>[2x]GADSVKIGFITDMSGLYADIDGQGGLEAIKMAVADFGGKVNGKPIEVVYADHQNKADIAASKAREWMDRGGLDLLVGGTNSATALSMNQVAAEKKKVYINIGAGADTLTNEQCTPYTVHYAYDTMALAKGTGSAVVKQGGKTWFFLTADYAFGKALEKNTADVVKANGGKVLG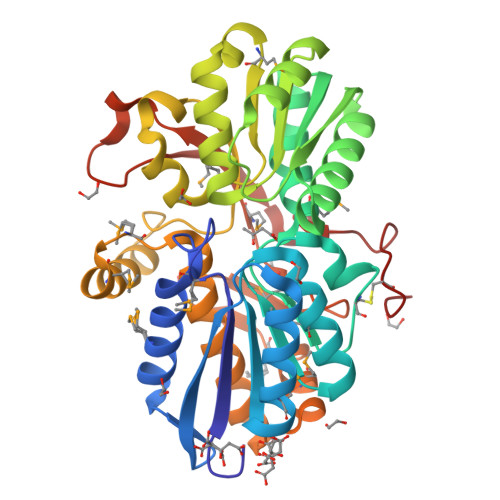EVRHPLSASDFSSFLLQAQSSKAQILGLANAGGDTVNAIKAAKEFGITKTMKLAALLMFINDVHALGLETTQGLVLTDSWYWNRDQASRQWAQRYFAKMKKMPSSLQAADYSSVTTYLKAVQAAGSTDSDKVMAQLKKMKIDDFYAKGYIRTDGSMIHDMYLMEVKKPSESKEPWDYYKVVATIPGEQAFTTKQETRCALWK>GPALNTEKMKTMLKAGMTVDDYAAKLKLTDKIAAAANSARAMEKLGETLKMKKLLRYLNYVAEHT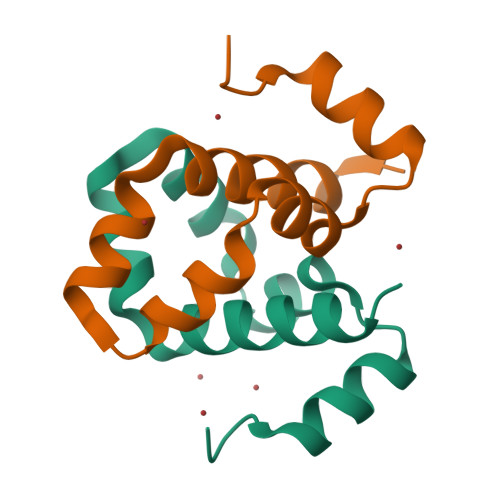AV[2x]> MRGSHHHHHHGSITSGNKSTNVTVHKSEAGTSSVFYYKTGDMLPEDTTHVRWFLNINNEKSYVSKDITIKDQIQGGQQLDLSTLNINVTGTHSNYYSGQSAITDFEKAFPGSKITVDNTKNTIDVTIPQGY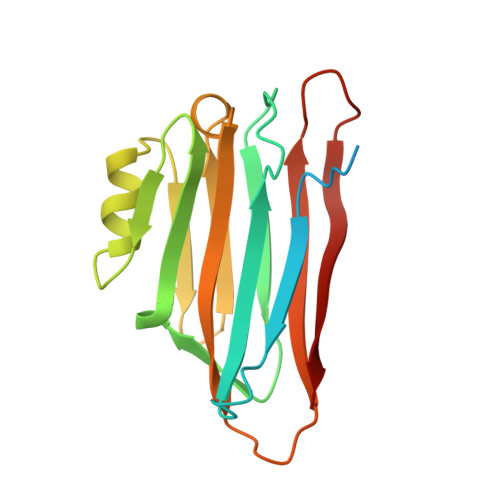GSYNSFSINYKTKITNEQQKEFVNNSQAWYQEHGKEEVNGKSFNHTVHN>[2x]SMGGKKFQAMPQLPSTVLDRVFEQARQQPEAIALRRCDGTSALRYRELVAEVGGLAADLRAQSVSRGSRVLVISDNGPETYLSVLACAKLGAIAVMADGNLPIAAIERFCQITDPAAALVAPGSKMAS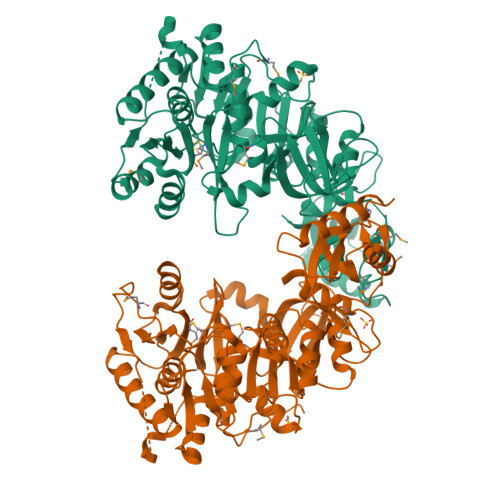SAVPEALHSIPVIAVDIAAVTRESEHSLDAASLAGNADQGSEDPLAMIFTSGTTGEPKAVLLANRTFFAVPDILQKEGLNWVTWVVGETTYSPLPATHIGGLWWILTCLMHGGLCVTGGENTTSLLEILTTNAVATTCLVPTLLSKLVSELKSANATVPSLRLVGYGGSRAIAADVRFIEATGVRTAQVYGLSETGCTALCLPTDDGSIVKIEAGAVGRPYPGVDVYLAATDGIGPTAPGAGPSASFGTLWIKSPANMLGYWNNPERTAEVLIDGWVNTGDLLERREDGFFYIKGRSSEMIICGGVNIAPDEVDRIAEGVSGVREAACYEIPDEEFGALVGLAVVASAELDESAARALKHTIAARFRRESEPMARPSTIVIVTDIPRTQSGKVMRASLAAAATADKARVVVRG>[2x]MAVPFVEDWDLVQTLGEGAYGEVQLAVNRVTEEAVAVKIVDMKRAVDCPENIKKEICILKMLNHENVIKFYGHRREGNIQYLFMELASGGSLFDRIEPDIGMPEPDAQRFFHQLMAGVVYLHGIGITHRDIKPHNLLLDERDNLKIADYSLATVFRYNNRERLLNKMCGTLPYVAP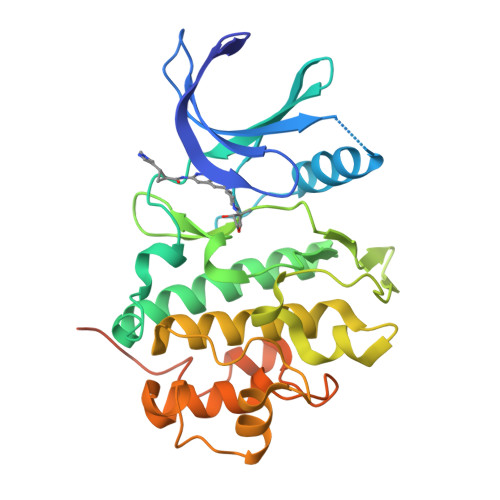ELLKRREFHAEPVDVWSCGIVLTAMLAGELPWDQPSDSCQEYSDWKEKKTYLNPWKKIDSAPLALLHKILVENPSARITIPDIKKDRWYNKPLKKGAKRPRVTSGGVSESPSGHHHHHHHH>SELDPKGQHVCVASSPSAELQCCAGWRQKDQECTIPICEGPDACQKDEVCVKPGLCRCKPGFFGAHCSSRCPGQYWGPDCRESCPCHPHGQCEPATGACQCQADRWGARCEFPSRHHHHHH[2x]

SCARF1 (scavenger receptor class F member 1, SREC-1 or SR-F1) is a type I transmembrane protein that recognizes multiple endogenous and exogenous ligands such as modified low-density lipoproteins (LDLs) and is important for maintaining homeostasis and immunity. SCARF1 (MW, 86 kD) is a type I transmembrane protein that has a short signal peptide followed by a long extracellular region, a transmembrane helix, and a large cytoplasmic portion (Adachi et al., 1997). Its ectodomain has three glycosylation sites and contains multiple EGF-like domains, which usually has a two-stranded β-sheet followed by a loop region and three conserved disulfide bonds. Here, we solve the crystal structures of the N-terminal fragments of human SCARF1, which show that SCARF1 forms homodimers and its epidermal growth factor (EGF)-like domains adopt a long-curved conformation.

Among them, two fragments (f1, 20–132aa and f2, 20–221aa) were crystallized and the crystals diffracted to 2.2 Å and 2.6 Å, respectively. The initial phasing for f1 crystal was done by SAD using Pt derivatives and the structure was refined to 2.2 Å with a native dataset after molecular replacement. The crystal of f1 fragment belongs to space group P212121 with two molecules per asymmetric unit. The f1 crystal structure contains a number of loops and two stranded β-sheets stabilized by hydrogen bonds and disulfide bonds, which is consistent with the typical feature of EGF-like domains, and it adopts a bow-like conformation with the middle part (~55–102aa) protruding outward. The electron density of the N-terminal end (~21–62aa) of one molecule in an asymmetric unit is relatively weak and some residues are missing, probably due to the flexibility of this region. In the crystal of f1 fragment, two molecules in an asymmetric unit are related by a twofold non-crystallographic symmetry axis. At the dimeric interfaces of f1 and f2 fragments, hydrogen bonds are formed between S88 and Y94 of the monomers, and F82 and Y94 are also close to each other, thus may form π-π interaction. Two salt bridges are also observed in f1 crystals between two monomers, one is between D61 and K71, the other is between R76 and D98. But the salt bridges are not found in f2 crystals, suggesting they are not required for dimerization. By contrast, mutant Y94A, where the hydrogen bonds and the π-π interactions between Y94 and F82 were both removed, showed a significant elution volume shift and the volume corresponded to the molecular weight of the monomeric SCARF1 ectodomain, suggesting that the π-π interactions between F82 and Y94 were important for dimerization.>MTMITHHHHHHGSSVQEFDPRNNVAPSMDALIGETPAVYLKRMNDTAATIVLKLECENPMASVKDRLAYAIYDKAEKEGKIIPGKSVIVEATSGNTGIALAHIGTIRGYKVIIVMPESMSIERRCLMRIFGAEVILTPAALGMKGALEAVNRIVSNNPDAVSANQFATKYNAQIHEETTGPEIWRQTKGHVDCFVAGVGTGGTITGVARYLKSVGCGATIFAVEPAESPVLSGGKPGPHRIQGIGAGFVPEVFEAALVDEVIQVSGDEAIDTAQKLPRTDGIFCGFSGGANVYAALQIAKRPEMAGKTIVTVIPSYGERYLSTALYSSIKDEVFALKVLSAADI[4x]

The de novo pathway of cysteine biosynthesis requires the conversion of O-acetyl-l-serine into l-cysteine, which is catalysed by cysteine synthase (CS). As CS is not found in humans, it constitutes a potential drug target. Crystal structures of the three enzymes were determined at resolutions of 1.80 Å for TcCS, 1.75 Å for LiCS and 2.75 Å for TthCS. These three homodimeric structures show the same overall fold and demonstrate that the active-site geometry is conserved, supporting a common reaction mechanism.

The protein crystallized with two independent dimers in the asymmetric unit, resulting in pseudosymmetry. Additionally, Thr188, Gly189, Thr191 and Ser275 all form hydrogen bonds to the ligand. In the active site of subunit A, additional density to the PLP was present. This density is fitted by O-acetyl-l-serine, an essential substrate of the cysteine-synthesis reaction. Lys52 and Asn83 both form hydrogen bonds to OAS. The reactive N atom of the OAS is 5.7 Å from the O atom of PLP that together form the Schiff base. Small molecules were found to be bound at the dimer interface of both TcCS dimers. Based on the unbiased electron density, ribose was identified in the AB interface, whereas glycerol was found in the CD dimer. The presence of these two molecules suggests that a hydrophilic pocket is formed at the dimer interface. In the presence of OAS this loop shows increased flexibility.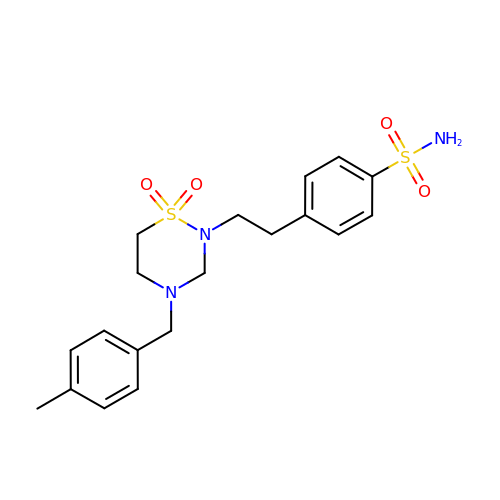4-[2-[4-[(4-methylphenyl)methyl]-1,1-bis(oxidanylidene)-1,2,4-thiadiazinan-2-yl]ethyl]benzenesulfonamide | C19 H25 N3 O4 S2 | RGMYFIVOQGMVRR-UHFFFAOYSA-N Like other TNF members, Eiger is a type II transmembrane protein with a single membrane-spanning helix, an intracellular portion, and an ectodomain harbouring the name-giving TNFα domain. Eiger activates the Jun N-terminal Kinase (JNK) signalling pathway by binding to its cognate TNF receptor. Two receptors of Eiger have been identified, termed Grindelwald and Wengen and which of these is utilized may be context and tissue specific. We crystallized the ectodomain of endogenous Eiger of S. frugiperda, an important agricultural pest which impacts food security, and solved its structure.

In this study we report the structure of the TNF domain of Spodoptera frugiperda Eiger (SfEiger) at 1.7 Å. We concluded that our structure constitutes the soluble SfEiger TNF domain (part of the Eiger ectodomain) which has been released from Sf9 cells into the culture medium. The domain is predominantly composed of β-strands organized into two β-sheets. The trimer resembles an inverted pyramid of ~60 Å height and ~50 Å width, with the β-sheet composed of strands A, H, C, and F forming the majority of the oligomerization interface. The interface between the three monomers is dominated by hydrophobic interactions. Several highly conserved residues, specifically His7, Leu71, Tyr73, Phe122, Phe154, and Val158 form the inner core of the oligomerization region. SfEiger possesses an additional α-helix located between strands A′ and B which is absent in EDA (indicated by a black arrow). Finally, the surface of the SfEiger trimer is decorated with a remarkable number of histidines (30 in total). Analysis of packing over multiple unit cells reveals sheets of SfEiger trimers which are aligned in a parallel fashion.

> RPFIAAHFHGNTSHLNSAIHDHYKGNGLVRVSHDAPHDVWYPAPWTVASPHPRPTLTRTGHVHVHHTGVYLVYVQIYYLDSHDTISWVLHRTNADIEGRETLLQCAQSSYSTEPIDKPNSCFSAAALFLKAGDRLAVRNTAGDRHSLMQPEKSFIGLVKLADAEDPTQEL> 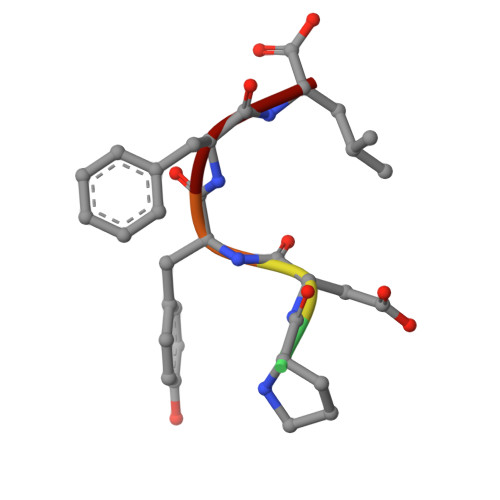TPDYFL As scaffold for implementing fold-switched allosteric assemblies, we chose chymotrypsin inhibitor 2 (CI2) from barley seeds. The small (<70 residues) globular single-domain CI2 is a paradigm of two-state folding in which a sturdy native structure unfolds at an extremely slow rate via an all-or-none transition. The CI2 native structure contains a four-stranded β-sheet and one α-helix connecting strands 1 and 2. The C-terminal β-strand is inserted in antiparallel fashion into the sheet’s middle, breaking an otherwise parallel arrangement to form a unique fold that is specific to this family of serine protease inhibitors.

To identify possible spatial arrangements for assembly, we analyzed the crystal lattice of CI2 by X-ray crystallography. CI2 crystallizes in the hexagonal space group P622 in all the conditions we attempted that rendered crystals. On the lattice, the protein forms double hexameric rings in which the two rings are packed head to head and rotated by ~30°. This spatial arrangement is strongly predefined by symmetry, and thus we identify the toroidal D6 particles of the crystal as the target for engineering a CI2 assembly. The lattice also reveals that inter-monomer contacts are few and feeble, both between ring neighbors and across rings (left), explaining why the protein is monomeric at all conditions outside the crystal. Indeed, crystals obtained using salt as primary precipitant follow the standard arrangement of early structural work on CI241 (left), whereas crystals grown with PEG feature domain-swapped dimers arranged in the same lattice structure and group symmetry (right). In solution, we find that CI2 is monomeric at concentrations up to the millimolar range and remains monomeric even after unfolding partially at high temperatures.

> DLKTEWPELVGKSVEEAKKVILQDKPEAQIIVLPVGTIVTMEYRIDRVRLFVDKLDNIAEVPRVG>[2x]MASSRRESINPWILTGFADAEGSFLLRIRKNNKSSVGYSTELGFQITLHNKDKSILENIQSTWGVGVIANSGDNAVSLKVTRFEDLKVIIDHFEKYPLITQKYADYMLFKQAFNVMENKEHLTIEGIKELVRIKAKLNWGLTDELKKAFPEIISKERSLINKNIPNFKWLAGFTSGEGCFFVNLIKSKSKLGVQVQLVFSITQHIRDKNLMNSLITYLGCGYIKKKNKSEFSWLDFVVTKF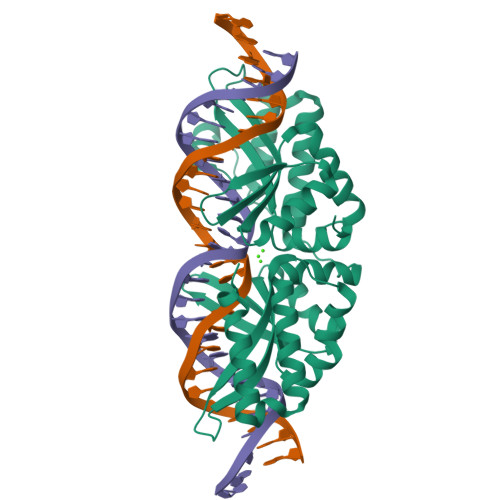SDIRDKIIPFFQEYTLIGTKLKDFEDWCKVAKLIEEKKHLTEEGLDEIKKIKLNMNKGRVF>[10x]NLIRKNVDTLTPDEILNLQVSLRAMQDDEGASGYQAISAYHGEPADCKAADGSTIVCCLHGMPTFPMWHRLYLVQFEQALVAHGSTLGIPYWDWTKPMTQLPELVQHPLFIDPTGKKAKKNVFYSGEIKFENKVTARAVDARLYQASQEGQKNFLLEGVLNALEQEDFCHFEVQLEVAHNPIHYLVGGRFTHSMSSLEYTSYDPLFFLHHSNVERHFALWQALQKHRGLPTRPNCGLNLFHSPMEPFGRDTNPFAITKDNSKASSLFDYEHLGYAFDDLSLNGMTIEELEALLKQRRSGARAFANFRLGGIKTSANVRIKLCIPTEDKRQSDNCDNDAGQFFILGGTNEMPWNFAFPYLHEITDTVLSLGLALDSNYYVTAEVTAINGTLMPTQTIPRPIVTYIPPQGFKDVNMVNMDTSSLRFRKDISSLTTEEEYELRVAMERFMSDKSINGYQALAEFHGLPAKCPRPDALNRVACCIHGMATFPHWHRLVVMQFENALFTRGSPIGVPYWDWTKPFTALPSLLADETYVDPYTKETKPNPFFKAPIEFLKAGVHTSRQIDERLFKQPSKGDHGFLYDGLSLAFE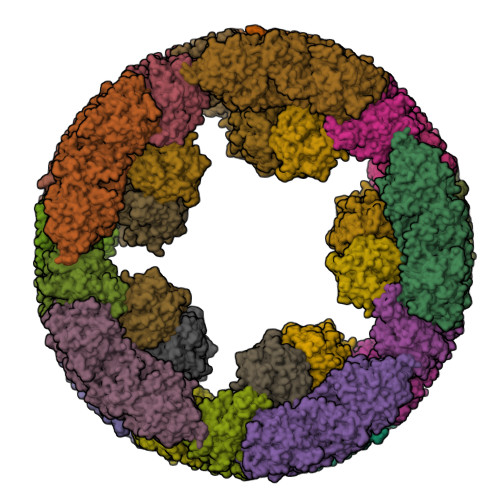QDDFCDFEVQFEVTHNSIHAWTGGSEPYSMSSLHYTSFDPMFWLHHSQVDRLWAIWQALQIQRGKPYKTYCANSEVYRPMKPFAFKSPLNNDEKTREHSVPTDVYDYQAELAYTYDTLFFGGLSIRELQRYVEEAKSKDRVFAGFLLMGIQTSANVDLFVVAGGNEFFVGSIAVLGGSKEMTWRFDRVYKHEITDALGALGVDMFAEYTLRVDIKDVNGTALPPTAIPPPIVIFVPGIADANVKFDEQHRSRKNVDSMTVSEMNALRTAMAAFAADKEVTGYQQVAAFHGSTQWCPSPDAAQKYACCHHGMATFPHWHRLIALNFENGLRRNGWSGGLPYWDWTRPIDALPALVLEAEYTDANGEAKPNPFFSGAIDSIGASTSRAPTEALYEKPDFGKYTHLANEIISALEQEDFCDFEVQYEIAHNHIHALVGGTEAVSMASLEYSAFDPIFMLHHSNVDRIWATWQALQKFRGKAYNSANCAIEILRKPMSPFSLASDINPDAMTREYSVPFDVFNYKKNFHYEYDTLELNGLSIAQLSREINRRKAKNRVAVTFMLEGLKKSLLVEYFIAADGTDQKMKAGEFYVLGSENEMPWKFDRPYKSDITYVMDAMKLHYTDKYHVELRITDMTGAEVTDLKLVTSVIYEPGIGNFGEGRRWISPITSASRIRKNLLDFEDGEMESLRNAFKQMADEGRYEEIASFHGVPAQCPSEDGTMVHTCCLHGMPVFPHWHRLYVSLVEDELLARGSGVAVPYWDWVEPFDELPRLINEATFYNSRTLQIEPNPFFKGKISFENAETDRDTQPELFGNRYLYDHTLFVFEQTDFCEFEVHYEVLHNTIHSWLGGRDVHSMSSLDYAAYDPVFFLHHSNVDRLWAIWQELQRYRKLSYNEANCALPLMNQPMRPFSNSTANNDRLTFTNSRPNDVFDYQNVLHYKYDTLNFAGLSIPQLERILQKNQGRDRIFAGFLLHGIKASADVRIYICVPTGIGEENCGNYAGIFSVLGGETEMPWQFDRLFRYEITDELKKLGLNQNSHFRVEMELTAVNGSKITQKIFPNPTIIFVPSDVEFEEDTWRDVVTSANRIRRNLKDLSKEDMFSLRAAFKRMTDDGRYEEIAAFHGLPAQCPNADGSNIHTCCLHGMPTFPHWHRLYLSLVENELLARGSDVAVPYWDWIEPFDSLPGLISDETYKHPKTNEDIENPFHHGKISFADAVTVRKPRDQLFNNRYLYEHALFAFEHTDFCDFEVHFEVLHNSIHSWIGGPNPHSMSSLDFAAYDPIFFLHHSTVDRLWAIWQDLQRYRKLDYNVANCALNLLNDPMRPFNNKTANQDHLTFTNSRPNDVFDYQNSLNYKFDSLSFSGLSIPRLDDLLESRQSHDRVFAGFWLSGIKASADVNIHICVPIGVEHEDCDN;>[10x]YAGTFAVLGGETEMPWAFDRLFRYEISDEMKKLQLTEDSKFRLTTNIIASNGSKVSNDIFPTPTVIFVPKKERTEQVSTTKSVRGNLVRKNVDRLSLQEINSLIHALKRMQKDRSSDGFETIASFHALPPLCPNPTAKHRHACCLHGMATFPQWHRLYVVQFEHSLNRHGAIVGVPYWDWTYPMTEVPGLLTSEKYTDPFTGIETFNPFNHGHISFISPETMTTREVSEHLFEQPALGKQTWLFNNIILALEQTDYCDFEVQFEIVHNSIHSWLGGKELYSLNHLHYAAYDPAFFLHHSNVDRLWVVWQELQKFRGLPAYESNCAIELMSQPLKPFSFGAPYNLNPVTTKYSKPSDVFNYKQNFHYEYDMLEMNGMSIAQLESYIRQERQKDRVFAGFLLEGFGSSAYATFQVCPDVGDCYEGSHFSVLGGSTEMPWAFDRLYKMEITDILQAMALKFDSHFTIKTKIVAHNGTELPESLLPEATIVRIPPSAQNLEVAIPLNRIRRNINSLESRDVQNLMSALKRLKEDESDFGFQTIAGYHGSLMCPTPEAPEYACCLHGMPTFMHWHRVYLLHFEESMRRHGASVAVPYWDWTMPSDNLPSLLGDADYYDAWTDSVIENPFLRGHIKYEDTYTVREIQPELFALAEGQKESTLFKDVMLMFEQEDYCDFEVQAEVIHNSIHYLIGGHQKYAMSSLMFSSFDPIFYVHHSMVDRLWAIWQELQKHRKLPHDKAYCALDQMAFPMKPFIWESNPNPTTRAVSTPSKLFDYKSLGYDYDHLNFHGMSIGQLEALIQKQKKADRVFAGFLLHGIKISADVHLKICIEADCQEAGVIFVLGGETEMPWHFDRNYKMDITDVLKKRNIPPEALFEHDSKIRLEVEIKSVDGAVLDPNSLPKPSLIYAPAKGLIIQQVGEYDAG;>SMVRKNVNSLTPSEIENLRNALAAVQADKTDAGYQKIASFHGMPLSCQYPDGTAFACCQHGMVTFPHWHRLYMKQMEDALKAKGAKIGIPYWDWTTAFHSLPILVTEPKNNPFHHGYIDVADTKTTRDPRPQLFDDPEQGDQSFFYRQIAFALEQRDFCDFEIQFEMGHNAIHSWVGGPSPYGMSTLHYTSYDPLFYVHHSNTDRIWAIWQALQKYRGLPYNSANCEINKLKKPMMPFSSEDNPNEVTKAHSTGYKSFDYQQLNYEYDNLNFHGMTIPQLEVHLKKIQEKDRVFAGFLLRAIGQSADVNFDVCRKDGECTFGGTFCVLGGDYEMPWAFDRLFLYDISKSLVHLRLDAHDDFDIKVTIMGIDGKSLPPNLLPSPTILFKPGTGKI[10x]>[2x]GHMWQENKSWNAHFTEHKSQGVVVLWNENKQQGFTNNLKRANQAFLPASTFKIPNSLIALDLGVVKDEHQVFKWDGQTRDIATWNRDHNLITAM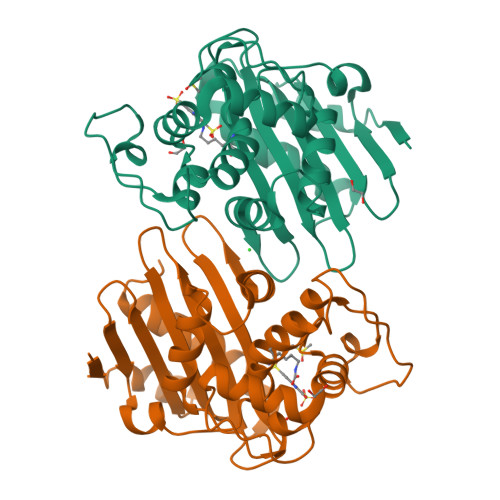KYSVVPVYQEFARQIGEARMSKMLHAFDYGNEDISGNVDSFWLDGGIRISATEQISFLRKLYHNKLHVSERSQRIVKQAMLTEANGDYIIRAKTGYSTRIEPKIGWWVGWVELDDNVWFFAMNMDMPTSDGLGLRQAITKEVLKQEKIIP> AVEQCDLSQFQTTSSNQLMAAIRQQGASCVNALFSADTGVQEAAFSSNHMYNVAQYTRTLAQQYAGGGSDELEALYLYLRAGYYAEFYNSNITFLSWVTPAVKGAVDAFVQNAHFYDNGDAHGKVLNEVIITMDSAGLQHAYLDVVTQWLTRWNAQYAEHWYMRNAVNGVFTLLFGGQWNNQYTSLIGEQTALVTALQAFALDRTKVNSPTEFMAANAARELGRLARYTDATIAPKVTEGLTAIFGQYPSYGDGDAIWLGAADTASYYADCSQFNICGFEDALRDAALNQTFICSDTIKIRSQDMSQA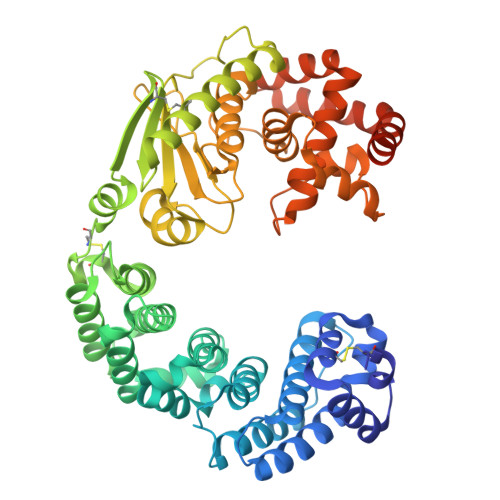QHLAACDKMAYEESFFHTTLETGNQPVADDHNTQLQVNIFNSDTDYGKYAGPIFGIDTNNGGMYLEGNPANVGNIPNFIAYEASYANPDHFVWNLEHEYVHYLDGRFNMYGDFGTPTELVVWWSEGVAEYVSRVNDNPQAIATIQDGSTYTLAQVFDTTYDGFDVDRIYRWGYLAVRFMFERHPDEVQRMLSATRQGRWAEYKAIISGWANQYQSEFAQWTEALAKGDSGAGNGEGTGSGNEGGGESGGNT>GPGSMASIFTKIINRELPGRFVYEDDDVVAFLTIEPMTQGHTLVVPREEIDNWQDVDSAAFNRVMGVSQLIG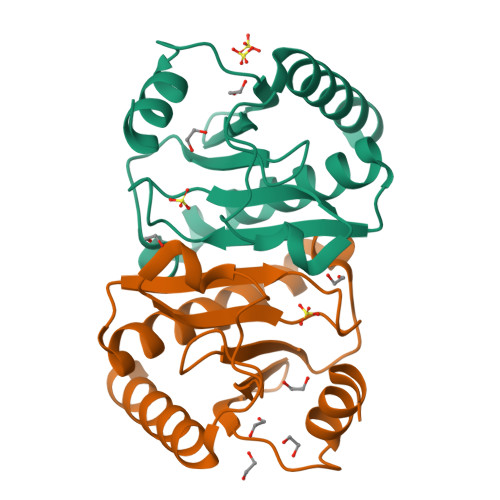KAVCKAFRTERSGLIIAGLEVPHLHVHVFPTRSLSDFGFANVDRNPSPESLDEAQAKIKAALAQLA[2x]>[5x]NAMIIRPEQHWFLRLFDWHGSVLSKIIFRLLLNVLMSIIAIISYQWYEQLGIHLTVAPFSLLGIAIAIFLGFRNSASYSRFVEARNLWGTVLIAERTLVRQLRNILPAEHDAHRRIVSYLVAFSWSLKHQLRKTDPTADLRRLLPEERVTEILASSMPTNRILLLAGNEIGQLREAGKLSDITYGLMDNKLDELAHVLGGCE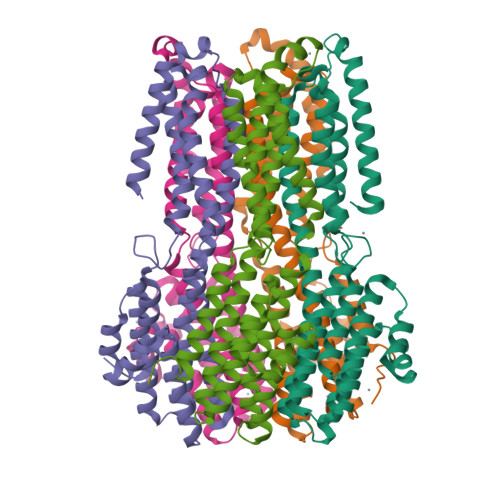RLATTPVPFAYTLILQRTVYLFCTLLPFALVGDLHYMTPFVSVFISYTFLSADSLAEELEDPFGTAANDLPLNAMCNTIERNLLDMTGQHPLPE> GSLDIAVYWGQSFDERSLEATCDSGNYAYVIIGFLNTFGGGQTPALDISGHSPKGLEPQIKHCQSKNVKVLLSIGGPAGPYSLDSRNDANDLAVYLHKNFLLPPAGTSESRPFGNAVLDGIDFHIEHGGPSQYQLLANILSSFRLSGSEFALTAAPQCVYPDPNLGTVINSATFDAIWVQFYNNPQCSYSASNASALMNAWKEWSMKARTDKVFLGFPAHPDAAGSGYMPPTKVKFSVFPNAQDSTKFGGIMLWDSYWDTVSQFSNKILGKGV

The XAIP-II and XAIP are two forms of a protein that possess two independent interaction sites and inhibits two structurally unrelated enzymes xylanase GH11 and α- amylase GH13. The polypeptide chain of XAIP-II adopts the triosephosphate isomerase (TIM) barrel folding with an eight stranded β-sheet that forms an inner circle while the nine α-helices constitute the outer loop. Because of the presence of an additional α-helix α8' (residues, 255-261) this protein is grouped in the subclass of family 18C proteins (GH18C) of the glycosyl hydrolases (GH 18) family. Hevamine also belongs to glycosyl hydrolase (GH) family 18C and has the characteristic combination of residues Asp125, Glu127 and Tyr183 for chitinase activity whereas the corresponding residues in XAIP-II are His124, Glu126 and Tyr182 indicating a loss of chitinase activity.

We have determined the structure of a new form of xylanase GH11 and α-amylase GH13 inhibitor protein (XAIP-II) at 1.2Ǻ resolution. The two forms, XAIP-II and XAIP show a sequence homology of 87% while 13% sequence variations occur mostly in the regions of ligand binding sites. The plateau line represents the steady state equilibrium phase of the interactions between the inhibitor and the enzymes whereas the decrease in RU from the plateau represents dissociation phase. As seen from Figures 2A and 2B, the dissociation phase is slower in the case of α-amylase than that of xylanase indicating a stronger interaction between XAIP-II and α-amylase GH13 (3.4 × 10-8 M) than that of XAIP-II and xylanase GH11 (4.2 × 10-6 M) as estimated using BIA evaluation software. The presence of Phe13 at the entrance of the channel in XAIP-II obstructs the entry of carbohydrates to the binding site. On the other hand, the presence of inwardly protruding Pro77 in the middle of the inner β-barrel blocks the channel passage right in the middle just before the positions of active site residues. As far as the differences between the impaired carbohydrate channels of XAIP-II and XAIP is concerned, the most notable variation is observed in the proximity of chitin binding site where Ala78 in XAIP-II has replaced Lys78 of XAIP. On the other hand, Ala78 in XAIP-II is oriented outwardly from the channel and hence does not exert any effect on the carbohydrate binding channel. The loop α3-β4 is considerably rigid in XAIP-II due to several intra loop interactions and hence lacks the freedom of getting induced fitting upon the binding of xylanase GH11. The insertion of an extra residue alanine at position 105 in the α3-β4 loop and replacements of His106 by Thr107 and Asn98 by Lys98 reduced both structural and chemical complementarities in XAIP-II with respect to the binding site in xylanase GH11 resulting in the formation of a less number of interactions with xylanase GH11.> MPFVNKQFNYKDPVNGVDIAYIKIPNAGQMQPVKAFKIHNKIWVIPERDTFTNPEEGDLNPPPEAKQVPVSYYDSTYLSTDNEKDNYLKGVTKLFERIYSTDLGRMLLTSIVRGIPFWGGSTIDTELKVIDTNCINVIQPDGSYRSEELNLVIIGPSADIIQFECKSFGHEVLNLTRNGYGSTQYIRFSPDFTFGFEESLEVDTNPLLGAGKFATDPAVTLAHELIHAGHRLYGIAINPNRVFKVNTNAYYEMSGLEVSFEELRTFGGHDAKFIDSLQENEFRLYYYNKFKDIASTLNKAKSIVGTTASLQYMKNVFKEKYLLSEDTSGKFSVDKLKFDKLYKMLTEIYTEDNFVKFFKVLNRKTYLNFDKAVFKINIVPKVNYTIYDGFNLRNTNLAANFNGQNTEINNMNFTKLKNFTGLFEHHHHHH;> RRATKMX

Seven antigenically distinct botulinum neurotoxins are produced by the bacterium Clostridium botulinum and they share considerable sequence homology, and structural and functional similarity. They are produced as inactive single chains of molecular mass 150 kDa and released as active dichains, a heavy chain (HC, 100 kDa) and a light chain (LC, 50 kDa) held together by an interchain disulfide bond. HC comprising two distinct domains is responsible for binding to neuronal cells and translocation into cytosol. LC is the catalytic domain cleaving one of the three proteins forming the SNARE complex (Soluble N-ethylmaleimide-sensitive fusion protein attachment protein receptors) required for docking and fusion of vesicles containing neurotransmitters to target cells. Catalytic domains of BoNTs are zinc proteases and cleave SNARE proteins with stringent substrate specificity though they share significant sequence similarity. BoNT/A and BoNT/E cleave the synaptosomal-associated 25 kDa protein (SNAP-25) while BoNT/B, /D, /F, and /G cleave the vesicle-associated membrane protein (VAMP).

In addition, we are also reporting the crystal structure of RRATKM, a variant of the substrate peptide, in complex with the enzyme. The crystal structure of Balc424 with a substrate analog RRATKM has been determined to 1.6Å resolution. The final refined model contains 423 residues of protease, 6 residues of substrate analog peptide, two sulfate ions, one zinc ion and 375 waters. The substrate analog could be modeled unambiguously in the residual map (Fo-Fc). Except for some minor variations of side chain orientations, the hexapetide RRATKM binds similar to the substrate peptide QRATKM. As in the case of QRATKM, the P1 (Arg197) amino group and the carbonyl oxygen chelate the catalytic zinc and the nucleophilic water has been replaced. P1-P5′ residues occupy identical subsites as in QRATKM. The only difference between QRATKM and RRATKM is at P1 residue. While P1-Gln197 makes a hydrogen bond with Glu164, P1-Arg197 makes a salt bridge interaction with Glu164 thus making it more strongly bound. The IC50 of QRATKM and RRATKM are 133 and 95 µM, respectively.>GGNSFVGLRVVAKWSSNGYFYSGKITRDVGAGKYKLLFDDGYECDVLGKDILLCDPIPLDTEVTALSEDEYFSAGVV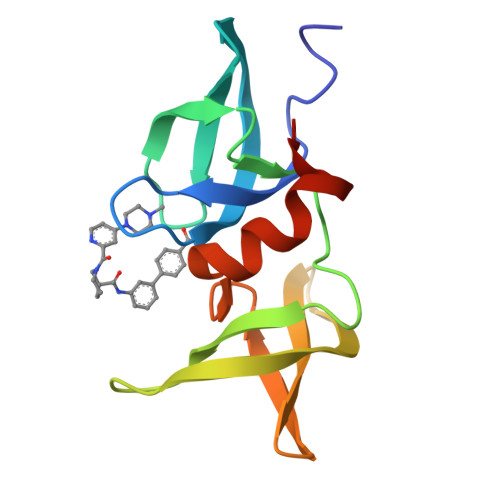KGHRKESGELYYSIEKEGQRKWYKRMAVILSLEQGNRLREQYGLGPYE[4x]>XGELAALKQELAALKWELAALKEELAAL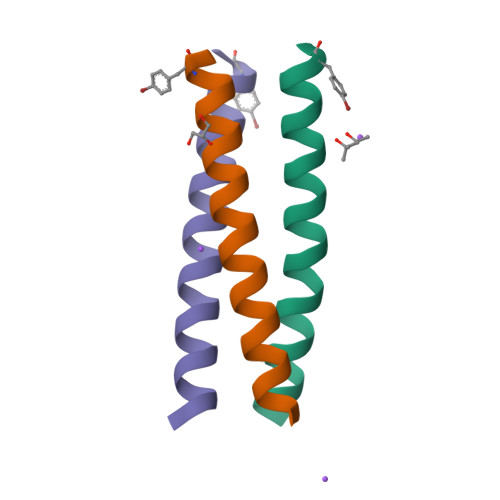KYGX[3x]>AMGYLWIRIPMAAAVIEEVEQRFSTPTALLRGIADAMVEEMERGLRADPHAPLKMLISYVDNLPTGDEHGLFYALDLGGTNFRVIRVQLGGREKRVVSQQYEEVAIPPHLMVGTSMELFDFIAAELESFVKTEGEDFHLPEGRQRELGFTFSFPVHQTSISSGTLIKWTKGFSINGTVGEDVVAELSRAMERQGLDMKVTALVNDTVGTLAGGRYVDNDVAAAVILGTGTNAAYVEHANAIPKWTGLLPRSGNMVINMEWGNFK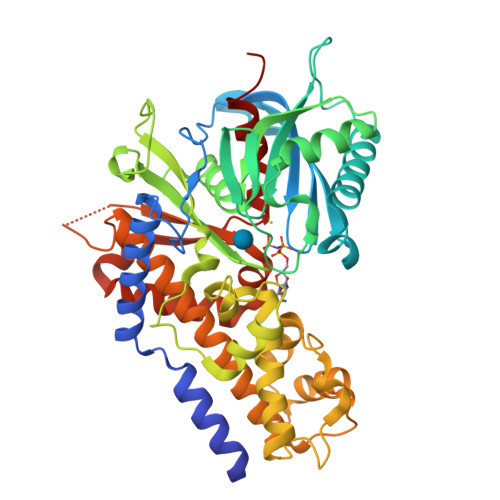SERLPRSDYDNALDFESLNPGEQIYEKMISGMYLGEIVRRILLKLAHDASLFGDVVPTKLEQRFILRTPDMSAMHHDTSHDLKHLGAKLKDILGVADTSLEARYITLHVCDLVAERGARLAAAGIYGILKKLGRDRVPSDGSQKQRTVIALDGGLYEHYKKFRTCLEATLADLLGEEAASSVVVKLANDGSGIGAALLAASHSQYASVE[3x]>WSHPQFEKENLYFQSMANVIKARPKLYVMDNGRMRMDKNWMIAMHNPATIHNPNAQTEFVEFPIYTVLIDHPEGKILFDTSCNPNSMGPQGRWAESTQQMFPWTATEECYLHNRLEQLKVRPEDIRYVVASHLHLDHAGCLEMFTNATIIVHEDEFNGALQCYARNQKEGAYIWADIDAWIKNNLQWRTVKRHEDNILLAEGVKVLNFGSGHAWGMLGLHVELPETGGIILASDAIYTAESYGPPIKPPGIIYDSLGYMNTVERIRRIAQETKSQVWFGHDAEQFKKFRKSTEGYYE[2x]

MLLs degrade N-acyl-L-homoserine lactones (AHLs), molecules that are used in a microbial communication system called quorum sensing (QS) to coordinate a variety of behaviors, including virulence and biofilm formation. We provide the structural and biochemical analysis of the lactonase GcL (WP_017434252.1), isolated from the thermophilic bacteria Parageobacillus caldoxylosilyticus. GcL is a thermostable, highly proficient lactonase with broad substrate specificity (kcat/KM values range between 104 to 106 M–1 s–1) for substrates such as N-butyryl (C4) L-homoserine lactone (HSL) and N-decanoyl (C10)-HSL. The binuclear center, common to all MLLs, is coordinated by five histidine residues and two aspartic acid residues.

GcL possesses a bimetallic active site center containing iron and cobalt cations. A water molecule bridges both metal cations, which has previously been hypothesized to be the reaction nucleophile in this family. The structure of GcL bound to C6-HSL (0.8 occupancy) is overall similar to the previously obtained structures of GcL bound to the substrates C4- and 3-oxo-dodecanoyl (3-oxo-C12)-HSL36. The lactone ring of the substrate sits on the bimetallic active site, with the carbonyl oxygen atom of the lactone ring interacting with the cobalt cation (2.6 Å) and the ester oxygen atom interacting with the iron cation (2.2 Å). In combination, these interactions likely increase the electrophilic character of the carbonyl carbon atom. The carbonyl oxygen atom is also hydrogen bonded to the hydroxyl group of Tyr223 (3.0 Å). The N-alkyl chain of C6-HSL is kinked and interacts with residue Ile237.> LLDPCGYISPESPVVQLHSNFTAVCVL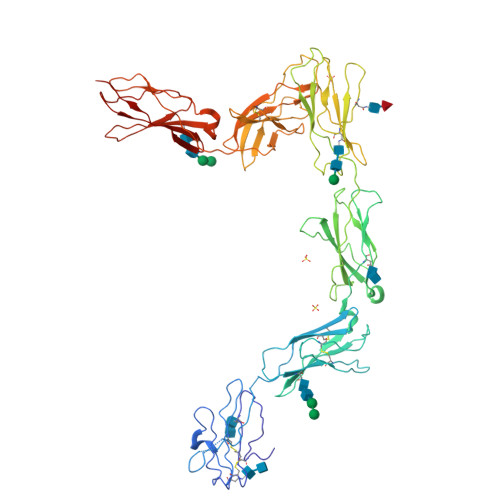KEKCMDYFHVNANYIVWKTNHFTIPKEQYTIINRTASSVTFTDIASLNIQLTCNILTFGQLEQNVYGITIISGLPPEKPKNLSCIVNEGKKMRCEWDGGRETHLETNFTLKSEWATHKFADCKAKRDTPTSCTVDYSTVYFVNIEVWVEAENALGKVTSDHINFDPVYKVKPNPPHNLSVINSEELSSILKLTWTNPSIKSVIILKYNIQYRTKDASTWSQIPPEDTASTRSSFTVQDLKPFTEYVFRIRCMKEDGKGYWSDWSEEASGITYEDRPSKAPSFWYKIDPSHTQGYRTVQLVWKTLPPFEANGKILDYEVTLTRWKSHLQNYTVNATKLTVNLTNDRYLATLTVRNLVGKSDAAVLTIPACDFQATHPVMDLKAFPKDNMLWVEWTTPRESVKKYILEWCVLSDKAPCITDWQQEDGTVHRTYLRGNLAESKCYLITVTPVYADGPGSPESIKAYLKQAPPSKGPTVRTKKVGKNEAVLEWDQLPVDVQNGFIRNYTIFYRTIIGNETAVNVDSSHTEYTLSSLTSDTLYMVRMAAYTDEGGKDGPEFTFTTPK> MVKYED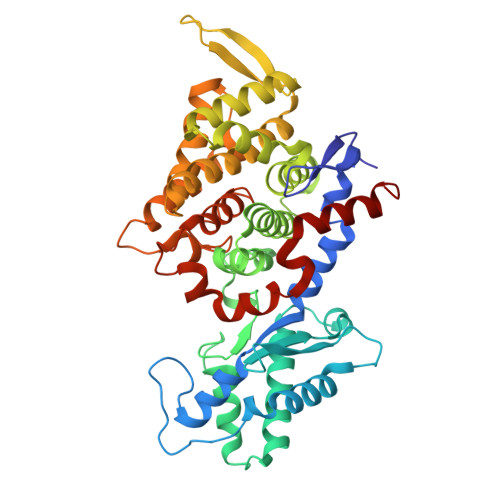KICLYNAKGELVEENVPLEAISPLYNPTIQKLVKDIKRTVAVNLAGIENALKTGAVGGKACVIPGRTLDLPIVENAETIMEYVDKLLRISPDDDTSVKLINDGKQMAVQLPSKRLEVAAEYSISMLNTAMALKEAIIKTFDVDMFDAPMVHAAILGRYPQVPDYMGANIASLLGAPTNLEGLGYALRNIMVNHYVATTKKNIMNAVAFASIMEQTAMFEMGDAIGSFERLHLLGLAYQGLNADNLVIDLVKANGKNGTVGTVVASIVERALEDGVITEDKKMPSGFVLYKPVDVAKWNAYAAAGLVAAVIVNCGAARAAQNVASTILYYNDIIEYETGLPGVDFGRAEGTAVGFSFFSHSIYGGGGPGIFNGNHIVTRHSKGFAIPPVCAAMCVDAGTQMFSPEKTSALVGAVFSAIDEFREPLKYVIDGALAVKDKI> ISMSSSEIIDVLCENLNDGIWALRVLYAEGAMNKEKLWDYINQYHKDYQIENEKDYEGKKILPSRYALDI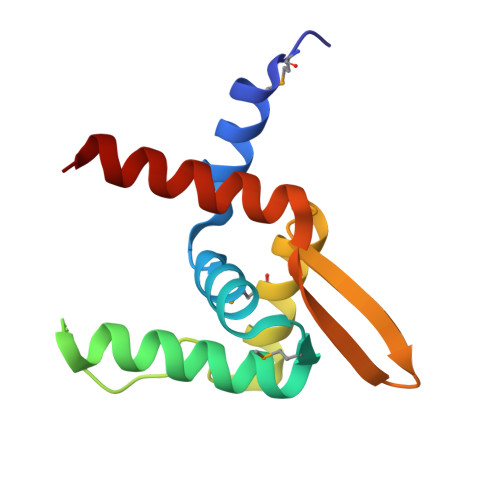MTARLEGAGLISFKAIGRVRIYDVTDLGNVLIKELEKRVEKNN>[2x]MGFL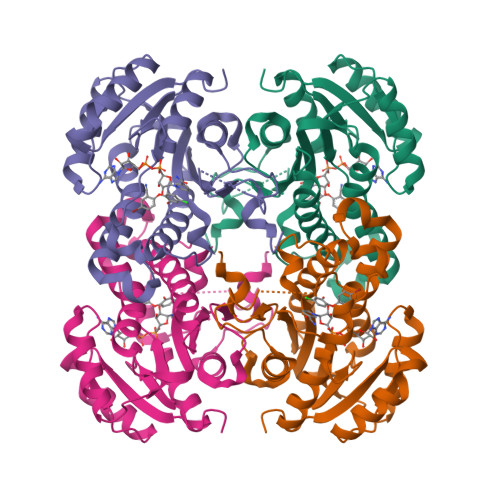SGKRILVTGVASKLSIAYGIAQAMHREGAELAFTYQNDKLKGRVEEFAAQLGSDIVLQCDVAEDASIDTMFAELGKVWPKFDGFVHSIGFAPGDQLDGDYVNAVTREGFKIAHDISSYSFVAMAKACRSMLNPGSALLTLSYLGAERAIPNYNVMGLAKASLEANVRYMANAMGPEGVRVNAISAGPIRTLAASGIKDFRKMLAHCEAVTPIRRTVTIEDVGNSAAFLCSDLSAGISGEVVHVDGGFSIAAMNELELKLEHHHHHH> MKTEWPELVGKSVEEAKKVILQDKPAAQIIVLPVGTIVAME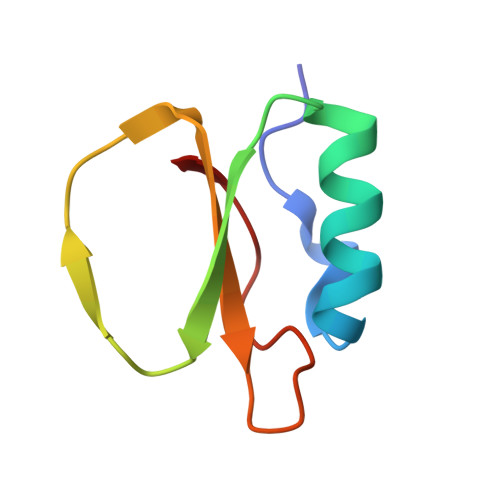YRIDRVRLFVDRLDNIAQVPRVG>MGLFDRIKRVVSSNLNDLVNKAEDPEKMLEQAILEMQEDLVQLRQGVAQAIAAQKRSEKQYNDAQNEINKWQRNAQLALQKGDENLARQALERKKTYTDTSAALKASLDTQSTQVETLKRNLIQLESKISEAKTKKEMLKARITTAKAQEQLQGMVRGMNTSSAMSAFERMEEKVLMQESRAQALGELAGADLETQFAQLEGGSDVDDELAALKAQMLPPATPVTQAQLPPQQETTPAKSNEVVDAELDSLRKQLDQL[90x]

Proteins that perform these functions include Vipp1/IM30 in photosynthetic plastids, PspA in bacteria, and ESCRT-III in eukaryotes. Here, using a combination of evolutionary and structural analyses, we show that these protein families are homologous and share a common ancient evolutionary origin that likely predates the last universal common ancestor. This homology is evident in cryo-electron microscopy structures of Vipp1 rings from the cyanobacterium Nostoc punctiforme presented over a range of symmetries. Rings have an inner lumen that is able to bind and deform membranes.

Reconstructions were also generated for the other six symmetries and complete ring models built. Rungs are maximally constricted at the top and bottom with internal lumen diameters of 14 nm and 15.7 nm, and widest at the ring equator between rungs 3 and 4 with an internal diameter of 17.5 nm. This unique asymmetric curvature is a feature of all Vipp1C11–C17 ring symmetries. The analysis of different ring symmetries, ranging from C11–C17, provides us with a view of the structural flexibility that enables Vipp1, PspA, and ESCRT-III family members to perform their functions. Furthermore, as each ring comprises between 5–7 rungs stacked together to build a dome-shaped architecture, these asymmetric structures provide us with a glimpse of the structural features that enable filament tilt in the context of an ESCRT-III-like polymer. Based on the Vipp1C11–C17 models, where helix α5C is positioned at the tip of the spike, α6 helices likely coat the ring outside surface and do not contribute directly to polymer formation. Consistent with this, Interfaces 1 and 3 linking the top two rungs were poorly resolved in Vipp1C11–C17 rings, indicating a weak interaction once the limiting geometry is reached. When membrane was modeled into the Vipp1C11–C17 structures as a 4-nm bilayer, sequential constriction was observed with the membrane lumen reaching ∼3 nm within Vipp1C11.6-(2-{2,3-difluoro-5-[3-(methylamino)prop-1-yn-1-yl]phenyl}ethyl)-4-methylpyridin-2-amine 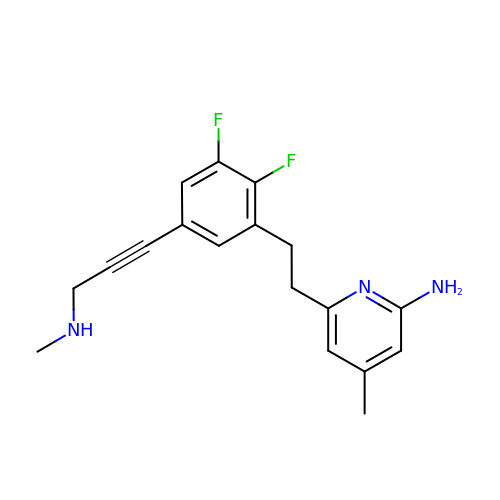| C18 H19 F2 N3 | VPIZCATWBQGZCY-UHFFFAOYSA-N2-[4-(3-chlorophenyl)piperazin-1-ium-1-yl]ethanenitrile 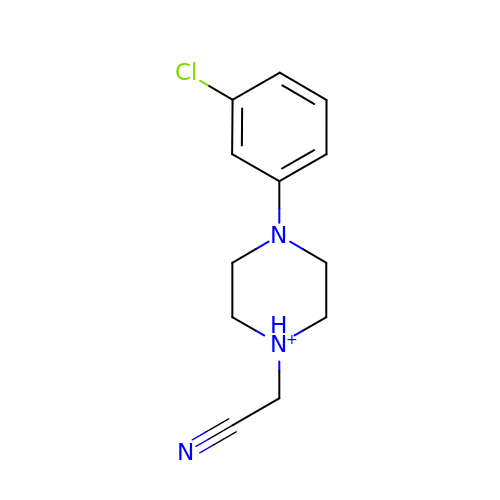| C12 H15 Cl N3 | BIGOTGAMVFQWPQ-UHFFFAOYSA-O>[3x]GSHMEEIKKQVQVNVDDIRAANIKLDGLGRQIADISNSISTIESRLGEMDNRLVGISSQVTQLSNSVSQNTQSISSLGDRINAVEPRVDSLDTVTSNLTGRTSTLEADVGS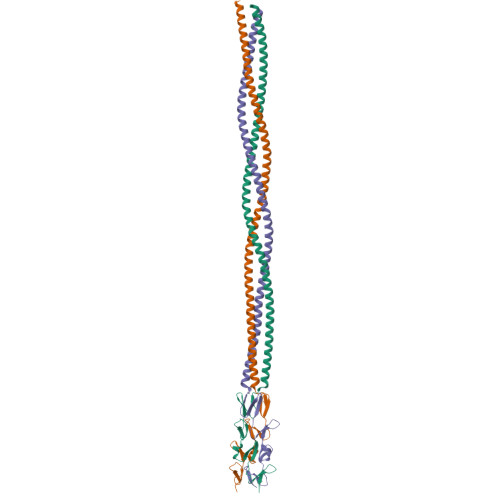LRTELAALTTRVTTEVTRLDGLINSGQNSIGELSTRLSNVETSMVTTAGRGLQKNGNTLNVIVGNGMWFNSSNQLQLDLSGQSKGVGFVGTGMVVKIDTNYFAYNSNGEITLVSQINELPSRVSTLESA(1~{R},2~{R})-cyclopentane-1,2-diol | C5 H10 O2 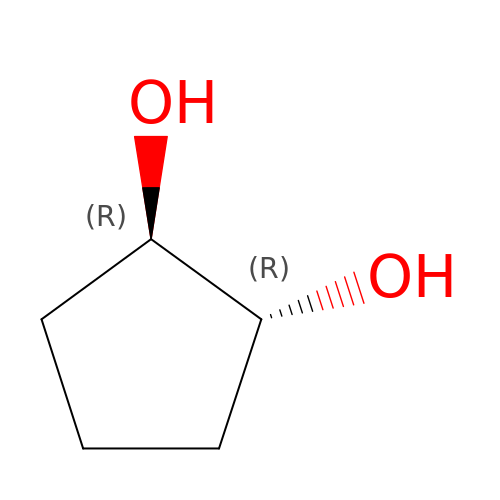| VCVOSERVUCJNPR-RFZPGFLSSA-N>[2x]MNYKELEKMLDVIFENSEIKEIDLFFDPEVEISKQEFEDLVKNADPLQKVVGDNYITETFEWWEFENQYLEFELDYYVKDEKIFVLEMHFWRKIRKLEHHHHHH;> MRNLKRIVMGENKLIGLVRTALDSITLGQGVNEAKIKSPQSYAFHTISVGTISLDICKAIYSSSEIGRKQLENLSKKYNMPFEDLWFYGGFLHDWNKLSGKEESLENKEELTKKIIDKLKLPNEFLHGISTMAEGHLPDNLHLPLWVSIKLADMLLISDIGSVRDVFYFANSDSYRNAIEALKEYNLELNYVSSTFRLFTLIASKELLNDVFNEKSGYFPLISYADGIVFLKRKNSQPVLLSKIVDLLSRQVFSSSSEVIEEKISDIEKCIKNKEELFRQMNID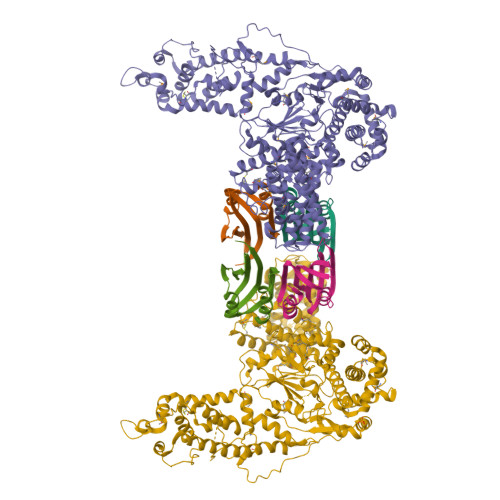VKSAIYDEEGKVKQINAFLPTKVCKPFEDVVGNLDNKSKLQVAREVIERNRKDIPFGLLIYFVNKFSKNEEDYIRKGLGINEKSLKYLLNIGDVQKALDKILELLEKRYAEQSSDKTLLYYVKFSSSGNIIDDLPKITDRPNDYCVVCGMPIYSSNPVRFVQYASELGGRAEIWIPREKALDEIDNVRDDWKVCPICIYEANLMKDRVKPPYFIVTFYPGVPISLLNIIDFDFSQSSIKYYIDEEKDTYFTAFEKMGGRLEPYVKKVLPAYFSSKVIIKASEVSNFSLSTRLSKSELNKLLPYAPMISMIFLTSPVLISSNLYEMPIAHERVISITSTYNYTFMKSLNSNLLTLYSIFAYSAKYDAMRKICGRSDLDNCLGYLTEEMDLYSSVDPALGVLSIGMGVGTPIDTDEKFFSAFLPVSGYLLKVTGKVSKMGETLKSSIFSIAYALKDIIKSQKVSKYDVTGFLRDGVDMFFKTTSVIKDKEDRIGISVNAAISSLENKYALDDQHRAQVYSALQDIFKTLYSIEEESDRSLAISIANTLSNWLYIAYKLVLQGDKSLEHHHHHH>MDKAELQKTLQANKIQGNIVSSSDLGSGLSMVIVEVNNQQAPFLATDDGKMIFQAEVLIAQDKSTESRVQEFYKNLYEKEKLRISAKLKEVFKAQKANVFTFKAKKPSNKTIYIVSDFNCPYCQREFANLDKRLESANVELLVVGFLGEDSILKAANALKNKSGNQAKDIAMLQKLYTPKSKGQSMDIKAAMALTQAVADTGVRSVPYII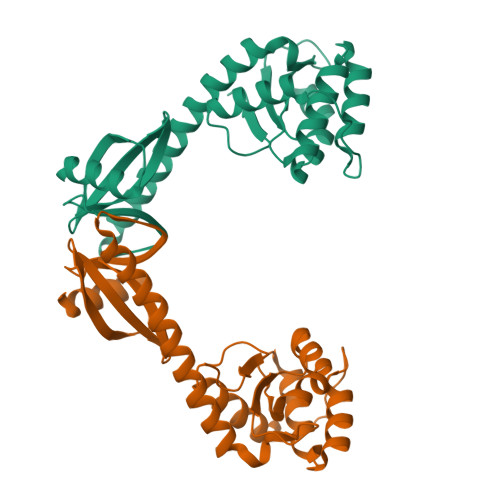EPHHHHHH[2x]> GPMDRYQRKIGCFIQIPNLGRGQLKYVGPVDTKAGMFAGVDLLANIGKNDGSFMGKKYFQTEYPQSGLFIQ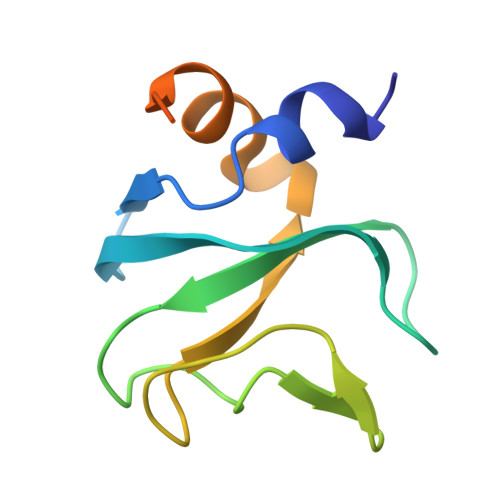LQKVASLIEKASISQTSRRTTMEPLSIPKNR>[2x]AKVLCVLYDDPVDGYPKTYARDDLPKIDHYPGGQTLPTPKAIDFTPGQLLGSVSGELGLRKYLESNGHTLVVTSDKDGPDSVFERELVDADVVISQPFWPAYLTPERIAKAKNLKLALTAGIGSDHVDLQSAIDRNVTVAEVTYCNSISVA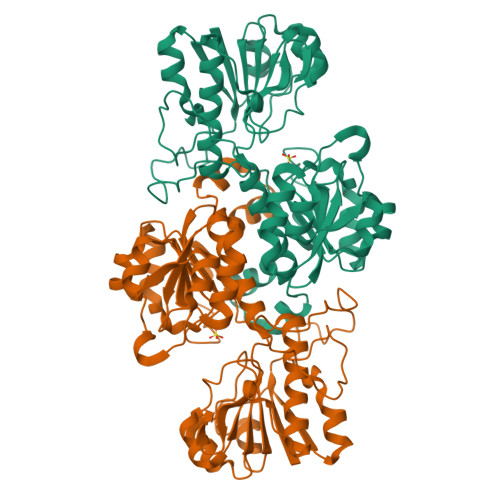EHVVMMILSLVRNYLPSHEWARKGGWNIADCVSHAYDLEAMHVGTVAAGRIGLAVLRRLAPFDVHLHYTDRHRLPESVEKELNLTWHATREDMYPVCDVVTLNCPLHPETEHMINDETLKLFKRGAYIVNTARGKLCDRDAVARALESGRLAGYAGDVWFPQPAPKDHPWRTMPYNGMTPHISGTTLTAQARYAAGTREILECFFEGRPIRDEYLIVQGGALAGTGAHSYSKGNATGGSEEA> SAYIEDFETKTRSTVSVREGQGVVLLCGPPPHFGELSYAWTFNDSPLYVQEDKRRFVSQDTGNLYFAKVEPSDVGNYTCFVTNKEAHRSVQGPPT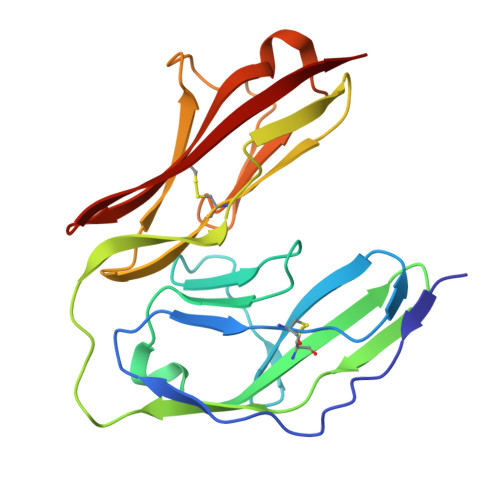PLVLRTDGVMGEYEPKIEVRFPETIQAAKDSSIKLECFALGNPVPDISWKRLDGSPMPGKIKYSKSQAILEIPKFQQEDEGFYECIAGNLRGRNLAKGQLIFYA>MGSSHHHHHHSQDPNSMSAVQPFIRTNIGSTLRIIEEPQRDVYWIHMHADLAINPGRACFSTRLVDDITGYQTNLGQRLNTAGVLAPHVVLASDSDVFNLGGDLALFCQLIREGDRARLLDYAQRCVRGVHAFHVGLGARAHSIALVQGNALGGGFEAALSCHTIIAEEGVMMGLPEVLFDLFPGMGAYSFMCQRISAHLAQKIMLEGNLYSAEQLLGMGLVDRVVPRGQGVAAVEQVIRESKRTPHAWAAMQQVREMTTAVPLEEMMR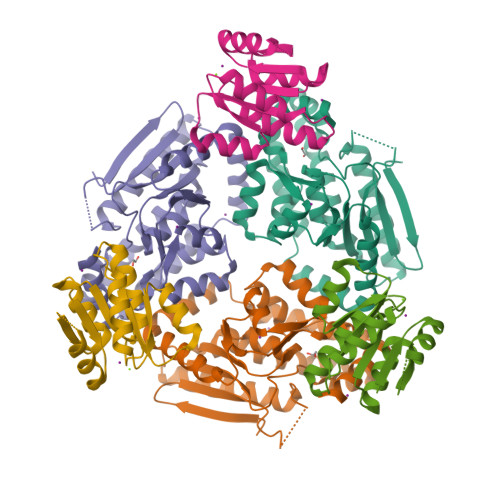ITEIWVDTAMQLGEKSLRTMDRLVRAQSRRSGLDAG[3x];>MSNPFLRHRARVRSMRMLVADDHEANRMVLQRLLEKAGHKVLCVNGAEQVLDAMAEEDYDAVIVDLHMPGMNGLDMLKQLRVMQASGMRYTPVVVLSADVTPEAIRACEQAGARAFLAKPVVAAKLLDTLADLAVSTRQLATP[3x]> GMTKIRKIAVFIEETRIEAGREISPPTRKAVAVAVIENPFAGRYVEDLTELMDTGAELGALLGERCVQALGIRPEQAESYGKSAM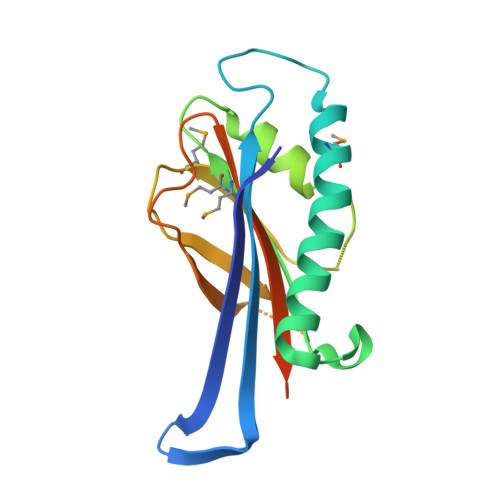VGENGELEHAAAILHPKLGAPLRKAVEKGAALVPSSKKMGSPGQVLDVPLGHKDAAYVRSHFDGIEVRLNDAPRANEIMVAVAVTDSGRPLPRVGGLTHDAAEGKDGLR>[3x]GPGMSTGGDFGNPLRKFKLVFLGEQSVGKTSLITRFMYDSFDNTYQATIGIDFLSKTMYLEDRTVRLQLWDT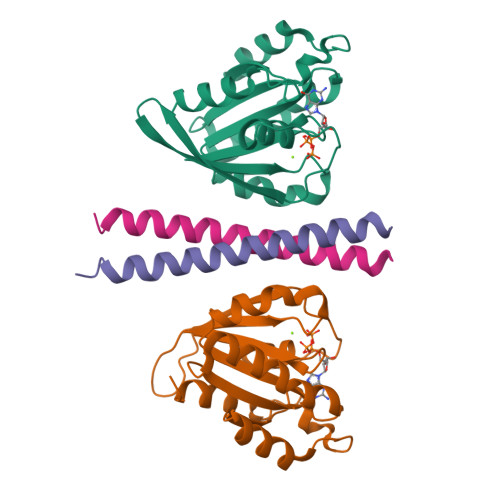AGLERFRSLIPSYIRDSTVAVVVYDITNVNSFQQTTKWIDDVRTERGSDVIIMLVGNKTDLADKRQVSIEEGERKAKELNVMFIETSAKAGYNVKQLFRRVAAALPGMESTQDRSREDMIDIKLEKPQEQPVSEGGCLL;>[3x]GPLGSLEPPLWHAEFTKEELVQKLSSTTKSADHLNGLLRETEATNAILMEQIKLLKSEIRRLERNQEREKS> KVVKFSYMWTINNFSFCREEMGEVIKSSTFSSGANDKLKWCLRVNPKGLDEESKDYLSLYLLLVSCPKSEVRAKFKFSILNAKGEETKAMESQRAYRFVQGKDWGFKKFIRRDFLLDEANGLL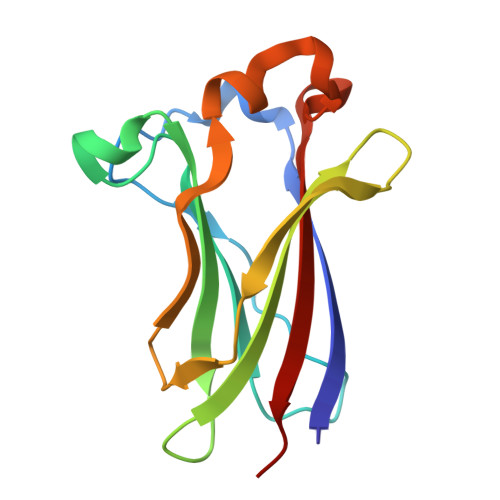PDDKLTLFCEVSVVQD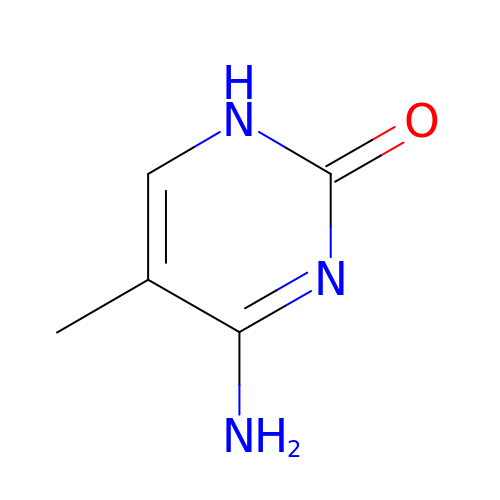5-methylcytosine | C5 H7 N3 O | LRSASMSXMSNRBT-UHFFFAOYSA-N> AAPGKPTIAWGNTKFAIVEVDQAATAYNNLVKVKN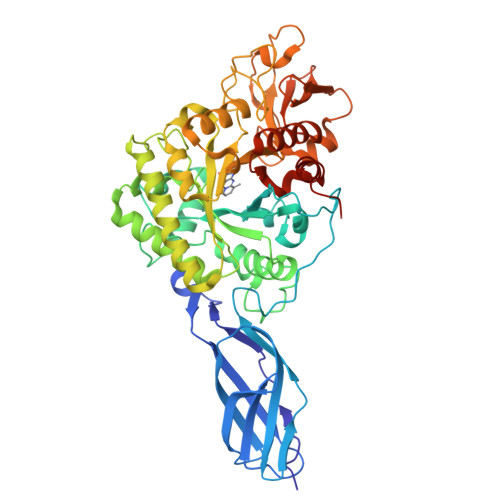AADVSVSWNLWNGDTGTTAKILLNGKEAWSGPSTGSSGTANFKVNKGGRYQMQVALCNADGCTASDATEIVVADTDGSHLAPLKEPLLEKNKPYKQNSGKVVGSYFVEWGVYGRNFTVDKIPAQNLTHLLYGFIPICGGNGINDSLKEIEGSFQALQRSCQGREDFKVSIHDPFAALQKAQKGVTAWDDPYKGNFGQLMALKQAHPDLKILPSIGGWTLSDPFFFMGDKVKRDRFVGSVKEFLQTWKFFDGVDIDWEFPGGKGANPNLGSPQDGETYVLLMKELRAMLDQLSAETGRKYELTSAISAGKDKIDKVAYNVAQNSMDHIFLMSYDFYGAFDLKNLGHQTALNAPAWKPDTAYTTVNGVNALLTQGVKPGKIVVGTAMYGRGWTGVNGYQNNIPFTGTATGPVKGTWENGIVDYRQIASQFMSGEWQYTYDATAEAPYVFKPSTGDLITFDDARSVQAKGKYVLDKQLGGLFSWEIDADNGDILNSMNASLGNSAGVQLEHHHHHH> GSSHHHHHHSSGLVPRGSMSTSWSDRLQNAADMPANMDKHALKKYRREAYHRVFVNRSLAMEKIKCFGFNMDYTLAVYKSPEYESLGFELTVERLVSIGYPQELLSFAYDSTFPTRGLVFDTLYGNLLKVDAYGNLLVCAHGFNFIRGPETREQYPNKFIQRDDTERFYILNTLFNLPETYLLACLVDFFTNCPRYTSCETGFKDGDLFMSYRSMFQDVRDAVDWVHYKGSLKEKTVENLEKYVVKDGKLPLLLSWMKEVGKVFLATNSDYKYTDKIMTYLFDFPHGPKPGSSHRPWQSYFDLILVDARKPLFFGEGTVLRQVDTKTGKLKIGTYTGPLQHGIVYSGGSSDTICDLLGAKGKDILYIGDHIFGDILKSKKRQGWRTFLVIPELAQELHVWTDKSSLFEELQSLDIFLAELYKHLDSS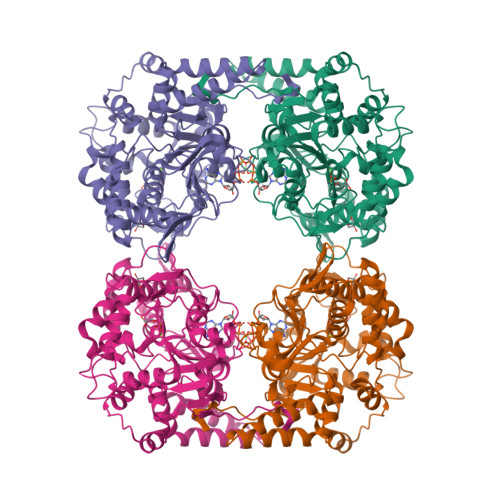SNERPDISSIQRRIKKVTHDMDMCYGMMGSLFRSGSRQTLFASQVMRYADLYAASFINLLYYPFSYLFRAAHVLMPHESTVEHTHVDINEMESPLATRNRTSVDFKDTDYKRHQLTRSISEIKPPNL> MRKFLKVTLASALIGCGVIGTVSSLMVKEAKAVEIITHWVPHEVYGMPGEPDNSGKVFFSGLKAKYMGYPKDAQRSPYPGKYSKFWKTLPAYRYYIPDYMYNRDEVRPSNPIKGTFKLEQCVACHSVMTPGIVRDYNKSAHSKAEPAPTGCDTCHGNNHQKLTMPSSKACGTAECHETQYNEQGQGGIGSHASCSSFAQVECAWSIERPPGDTAGCTFCHTSPEERCSTCHQRHQFDPAVARRSEQCK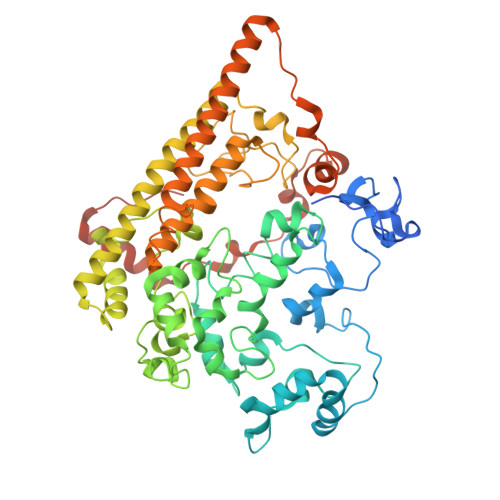TCHWGKDHRDWEAYDIGLHGTVYQVNKWDTEQFDFSKKLSDADYVGPTCQYCHMRGGHHNVQRASIVYTSMGMSMADRGAPLWKEKRDRWVSICDDCHSPRFARENLQAMDESVKDASLKYRETFKVAEDLLIDGVLDPMPKDLCPDWSGQHIWSLKIGAYHDGEAYGGTTGESGEFRMSNCTDVERLCFESVGYFQTYIYKGMAHGSWNDATYSDGSFGMDRWLVNVKQNASRARRLAALEKKVGISWQPEQFWKTGEWLDQLTGPYIVKNHPGKTIFDLCPDPGWLDTHHAPAEEVEYIERKLKELGITAGSHSAHHHESGHDPAARSMKEH1-({3-[(3R,5R)-5-(4-fluorophenyl)oxolan-3-yl]-1,2,4-oxadiazol-5-yl}methyl)-7-methyl-1,7-dihydro-6H-purin-6-one 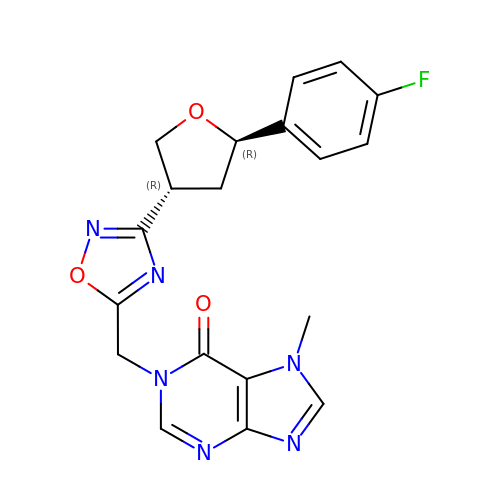| C19 H17 F N6 O3 | KVSPYEYQFMGJNK-GXTWGEPZSA-N> GAPQEVNSELPPLTIDGIPVSVDKMTQAQLRAFIPEMLKYSTGRGKPGWGKESCKPIWWPEDIPWANVRSDVRTEEQKQR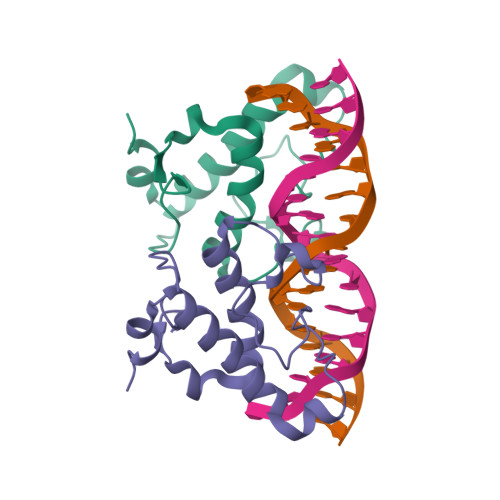VSWTQALRTIVKNCYKQHGREDLLYAFED>[2x]DYKDDDDKAAAQSLEFNSPADNYTVCEGDNATLSCFIDEHVTRVAWLNRSNILYAGNDRWTSDPRVRLL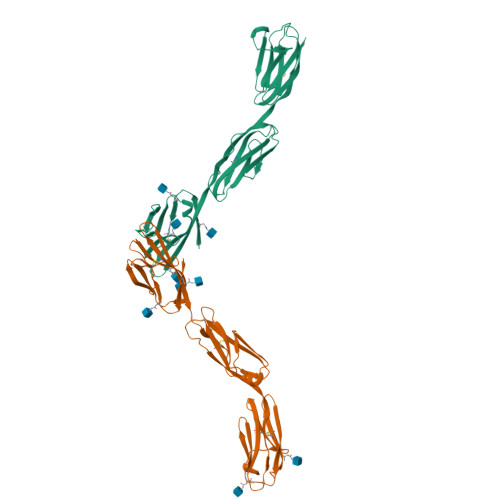INTPEEFSILITEVGLGDEGLYTCSFQTRHQPYTTQVYLIVHVPARIVNISSPVTVNEGGNVNLLCLAVGRPEPTVTWRQLRDGFTSEGEILEISDIQRGQAGEYECVTHNGVNSAPDSRRVLVTVNYPPTITDVTSARTALGRAALLRCEAMAVPPADFQWYKDDRLLSSGTAEGLKVQTERTRSMLLFANVSARHYGNYTCRAANRLGASSASMRLLRPGSLENSALEVLFQ> MSLKQTVYIASPESQQIHVWNLNHEGALTLTQVVDVPGQVQPMVVSPDKRYLYVGVRPEFRVLAYRIAPDDGALTFAAESALPGSLTHISTDHQGQFVFVGSYNAGNVSVTRLEDGLPVGVVDVVEGLDGCHSANISPDNRTLWVPALKQDRICLFTVSDDGHLVAQDPAEVTTVEGAGPRHMVFHPNEQYAYCVNELNSSVDVWELKDPHGNIECVQTLDMMPENFSDTRWAADIHITPDGRHLYACDRTASLITVFSV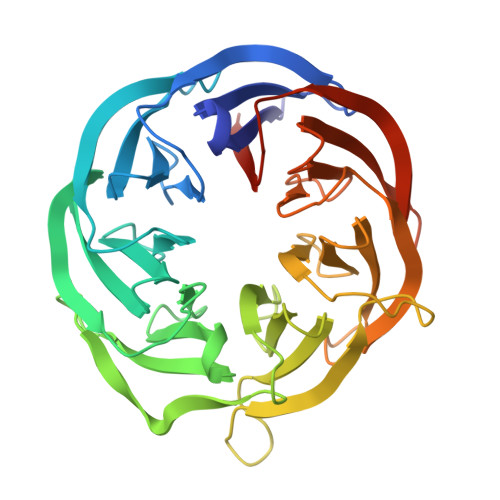SEDGSVLSKEGFQPTETQPRGFNVDHSGKYLIAAGQKSHHISVYEIVGEQGLLHEKGRYAVGQGPMWVVVNAHEGGSHHHHHH> AQVLRGTVTDFPGFDGRADAETLRKAMKGLGTDEESILTLLTSRSNAQRQEISAAFKTLFGRDLLDDLKSELTGKFQKLIVALMKPSRLYDAYELKHALKGAGTNEKVLTEIIASRTPEELRAIKQVYEEEYGSSLEDDVVGDTSGYYQRMLVVLLQANRDPDAGIDEAQVEQDAQALFQAGELKWGTDEEKFITIFGTRSVSHLRKVFDKYMTISGFQIEE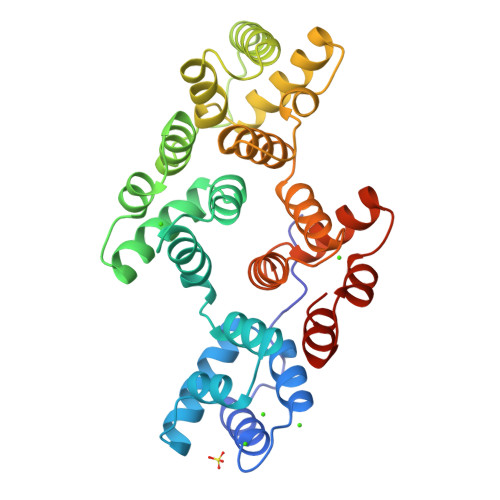TIDRETSGNLEQLLLAVVKSIRSIPAYLAETLYYAMKGAGTDDHTLIRVMVSRSEIDLFNIRKEFRKNFATSLYSMIKGDTSGDYKKALLLLCGEDD>MIERLNSPFLRAAALFTIVAFSSLISTAALAENNPSDTAKKFKVVTTFTIIQDIAQNIAGDVAVVESITKPGAEIHDYQPTPRDIVKAQSADLILWNGMNLERWFEKFFESIKDVPSAVVTAGITPLPIREGPYSGIANPHAWMSPSNALIYIENIRKALVEHDPAHAETYNRNAQAYAEKIKALDAPLRERLSRIPAEQRWLVTSEGAFSYLAKDYGFKEVYLWPINAEQQGIPQQVRHVIDIIRENKIPVVFSEST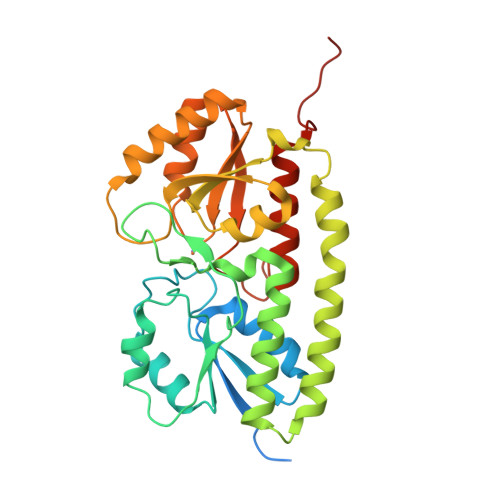ISDKPAKQVSKETGAQYGGVLYVDSLSGEKGPVPTYISLINMTVDTIAKGFGQLEHHHHHHHHHH[2x]>[2x]MASWSHPQFEKGASLDSPTFGCTDSPVRRERGQKAVFCGLTSIVWLHRKMQDAFFLVVGSRTCAHLLQAAAGVMIFAEPRFGTAVLEEQDLAGLADAHKELDREVAKLLERRPDIRQLFLVGSCPSEVLKLDLDRAAERLSGLHAPHVRVYSYTGSGLDTTFTQGEDTCLAAMVPTLDTTEAAELI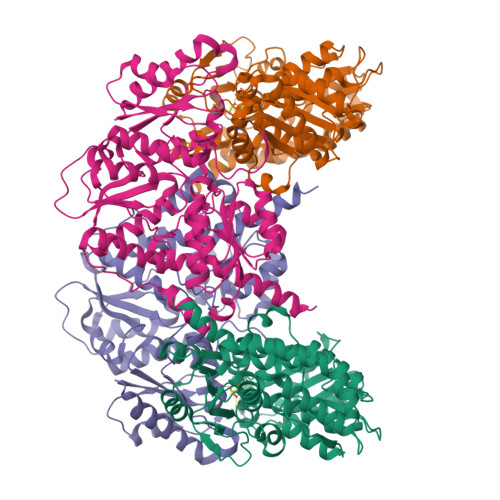VVGALPDVVEDQCLSLLTQLGVGPVRMLPARRSDIEPAVGPNTRFILAQPFLGETTGALERRGAKRIAAPFPFGEEGTTLWLKAVADAYGVSAEKFEAVTAAPRARAKKAIAAHLETLTGKSLFMFPDSQLEIPLARFLARECGMKTTEIATPFLHKAIMAPDLALLPSNTALTEGQDLEAQLDRHEAINPDLTVCGLGLANPLEAKGHATKWAIELVFTPVHFYEQAGDLAGLFSRPLRRRALLNGGAA;>MKLTLWTYEGPPHVGAMRVATAMKDLQLVLHGPQGDTYADLLFTMIERRNARPPVSFSTFEASHMGTDTAILLKDALAAAHARYKPQAMAVALTCTAELLQDDPNGISRALNLPVPVVPLELPSYSRKENYGADETFRALVRALAVPMERTPEVTCNLLGATALGFRHRDDVAEVTKLLATMGIKVNVCAPLGASPDDLRKLGQAHFNVLMYPETGESAARHLERACKQPFTKIVPIGVGATRDFLAEVSKITGLPVVTDESTLRQPWWSASVDSTYLTGKRVFIFGDGTHVIAAARIAAKEVGFEVVGMGCYNREMARPLRTAAAEYGLEALITDDYLEVEKAIEAAAPELILGTQMERNIAKKLGLPCAVISAPVHVQDFPARYAPQMGFEGANVLFDTWVHPLVMGLEEHLLTMFREDFEFHDAAGASHHGGKAVAREESPVAPADLAPAATSDTPAAPSPVVVTQASGEIRWMPEAERELRKIPFFVRGKAKRNTELYAAHKGVCDITVETLYEAKAHYAR[2x]Cefepime (open) | 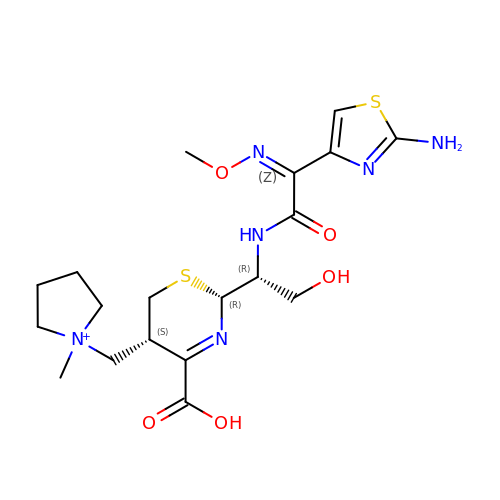C19 H29 N6 O5 S2 | XJYXJMZNAZABOJ-BNWKVGSUSA-O> MNNSKIISKVLLSLSLFTVGASAFVIQDELMQKKHAKAEVSAEEIKKHEEKWNKYYGVNAFNLPKELFSKVDEKDRQKYPYNTIGNVFVKGQTSATGVLIGKNTVLTNRHIAKFANGDPSKVSFRPSINTDDNGNTETPYGEYEVKEILQEPFGAGVDLALIRLKPDQNGVSLGDKISPAKIGTSNDLKDGDKLELIGYPFEHKVNQMHRSEIE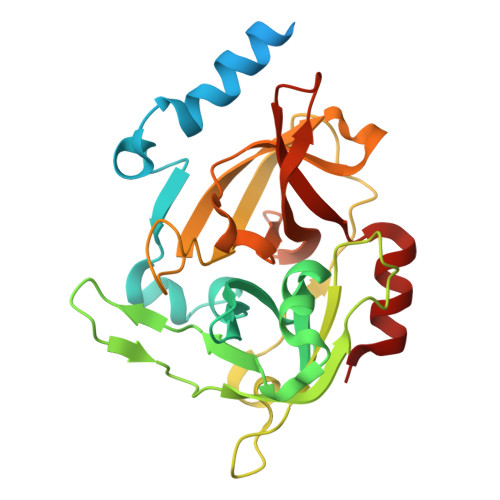LTTLSRGLRYYGFTVPGNSGSGIFNSNGELVGIHSSKVSHLDREHQINYGVGIGNYVKRIINEKNE Here, we report cryo-EM structures of the core DISARM complex, DrmAB, both alone and in complex with an unmethylated phage DNA mimetic. The DrmAB complex exhibits a bi-lobed architecture, resembling a partially open clam shell. The top lobe contains the RecA1 domain of DrmA, while the bottom lobe contains the DrmA RecA2 domain and the entirety of DrmB. As expected for a superfamily 2 (SF2) helicase, DrmA contains tandem RecA modules (residues 600–1150) that form an active site for ATP-binding and hydrolysis and DNA loading.

Two dominant, distinct populations (~120,000 particles each) emerged during focused 3D classification; one of which had strong DNA density (DrmAB:ADP:DNA) and one lacking observable DNA density (DrmAB:ADP). Notably, we were able to separate DNA-bound from DNA-free particles through focused 3D classification, ultimately yielding 3D reconstructions of DrmAB:ADP:DNA and DrmAB:ADP at nominal resolutions of 3.3 and 3.4 Å, respectively. We observed strong density corresponding to ADP within our DNA-bound and DNA-free maps, both of which were at the interface between the RecA1 and RecA2 domains, the canonical ATP-binding site of SF2 helicase domains. Comparison of our two maps revealed the presence of a 55-residue loop in DrmA that is otherwise absent in the DNA-bound structure. Due to the flexibility of this loop, we were unable to confidently assign sequence position. We modeled this region as poly-alanine. Thus, the presence of this loop is mutually exclusive with DNA binding. Given that the presence of TL and DNA are mutually exclusive, we hypothesized that in the absence of single-stranded DNA, this loop may partially occlude the DNA binding site, preventing DrmAB from loading onto non-phage (i.e., host) DNA. In the absence of DNA, the DNA-binding channel of DrmAB is occluded by an unstructured ~50 residue loop within TL. I In the absence of phage infection, DrmAB complex is autoinhibited via TL.

> MTDNNKSSKTPNAWIAIDHNFSRAQVLTYYTLQLKGEHSLHQAISDNDWILVLDTTGNITRVGRILRIRSDLETTTIFFDRMLQVKSVVSIGITPFKFPPNDRAGRIQWTDFIETLPKELHITIADIPKIEDQTYIRELLQLAVMDDLLGPAGGPNELIVDMGVRDRYLVGKLAPREAAERGQEFPIDAEDIEDEEPDLIVKAKTAKVNSPSVLGSGETDTAEEIDAASNQSLVPSSLGMTFCVDGDVDRVEIEARWGRYERVPNDEHQFFKSNGQKAKVWKRIPCGGKIVLPLIEGSISHNAPDSTSPEVRVQGSIRAKNDNGDRLITLFLVNAQEEPDTNRDTAWVFQPELIVRAAKDAAKPAIFRRRPVLDADGMDPEREALEMIYRDRVEFAVGHGVAVHAEIADDVTLATEVRTTVMPQYEVQATETPGLELSDRPAMREMVSSGLLDMQRLATLDIDPLVDALSVLTNDYATWIDEQNLNVSSKAKGFDTQAQTAINRCQEIHTRLQEGINTLKSNENALAAFRFANQAMATQRIRSLYALAMRRGEDVTLDKFDVLKNRSWRPFQLAFLLLSIPSLADPCHPDRVKPIEAYADLLWFPTGGGKTEAYLGVAAFTMAIRRMQGNLGGYDSSRGLTVIMRYTLRLLTLQQFQRATALICAMEVLRREALNKGDKSLGTEPFTIGLWVGNKVTPGTTEDSHNAIEKTRNPGSYNAGTASPVQLTSCPWCGTEIVPGQDVEVKKDKAGGRTFVYCGDKKGRCEFSKGKSSTQPHPGIPVLVVDEEIYHRPPTMMIATVDKFAMMAWRGQVRTLFGRVEKECERHGLLWPGANCTGNHQAFKGQPSAKVKAIPPIRPPDLIIQDEFHLISGPLGTMVGLYETAVDELCSWTLNGKTVKPKIIASTATVRKAKEQVNNVFMRQVSVFPPHGLDVEDNFFSVQRHIKDKFGRRYLGVCSPGSSRPAMLIRVYTAFLTAAQELFDHFGEPADPYMTMVGYFNSLRELGGMKRLAEDDVQTRSYRVQMSMVERPALAQRSVNNIRELTSRVSSQDIPKYLDNLEVKFKAEFDSSAGKYVTKWQEGDTRAIDVVLATNMLSVGVDVNRLGLMAVNGQPKGTAEYIQATSRVGRSFPGLVCTVLTWARPRDLSHYETFEHYHATFYKHVEAQSVTPFSPRAMDRGLTGSLLSLMRLKNNEFSPNEGAGKLDMSNQSELAHAIEVLATRAGNVAEDNARKLLAENELKERADEWAKEASKGGRILGYEKRGPDKDKTVALIKSPGLQAWDNWTVPMSMREVESGVRLIMDTKFIKDDHDWKPRPATKDED;> MIINNKTPVGEVRPSQLLWTYGPGALIDLPSLSVVTLGIDRWERERCQPIQEARLLAAVRKVLGPQVENLRMPPFQKSELVDPWSAEANIGVPVRPFPRWMRCVKCGLLSPFDDGLLEIKEDRFRAERTRFVHKGCTGSKGNLPAKDADAVPARFLLACRDGHLDDFPWHYFVHGGNSTCKGTLRFFESGASLQTENLWVRCDSCEASRSMAHAFGKAGKENLPACRGRHPHLDQFDIDCGEEPRAVLLGATNSWFPITLSALAIPQSKNPLSQLIQDGWPLFEAITAEVMVPIVVQTLKLTGGLPGIDKYSVSDIWSAIEMHRSGGDSEFVGEADIKGPEWEVLTEANPPTDYPHFMSKKIGTPAQFIPYISRVLLLERLREVNALLGFTRVEAPEGSGEINERPQMASLARNKPEWVPANQVHGEGIFIQFNEKTLVAWESLDAVKQVDEMLRGGHTGWRNSRNLDPNEDYPGIRYAMLHTLSHLLIRELALECGYNAASIRERIYADTSNGSPQAGILIYTAAADSDGTLGGLVDLGKPENLGRLLVQALNRSKICSSDPLCSEHNPEKDRSLHAAACHACTLVAETSCEQGNRYLDRSLLIPTLERIHAAFFKGF> MGSDKIH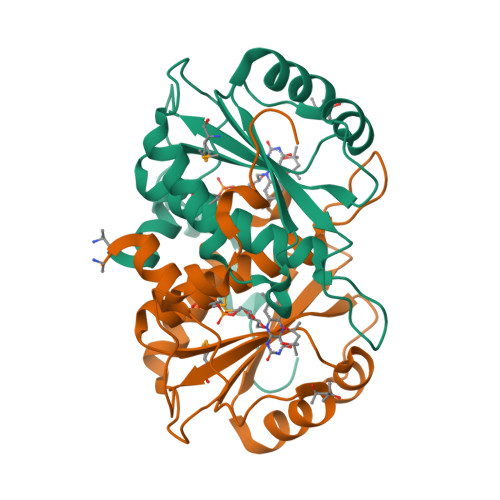HHHHHENLYFQGMNFVELAKKRYSCRNYQDRKVEKEKLEKVLDVARIAPTGGNRQPQRLIVIQEKEGINKLSKAANIYDAPLAILVCGDKDKVWTRPFDGKQLTDIDTSIVTDHMMLQATELGLASVWVCYFNPDIIREEFSLPDNLEPINILLMGYESKIPESPERHEKTRVPLSEIVSYETL> RR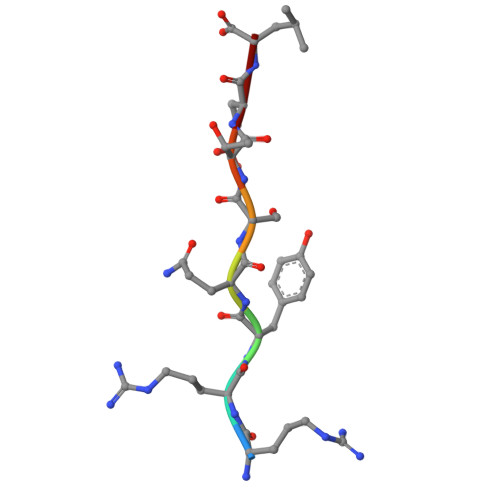YQSTEL>[3x]GVLMDEGAVLTLAADLSSATLDISKQW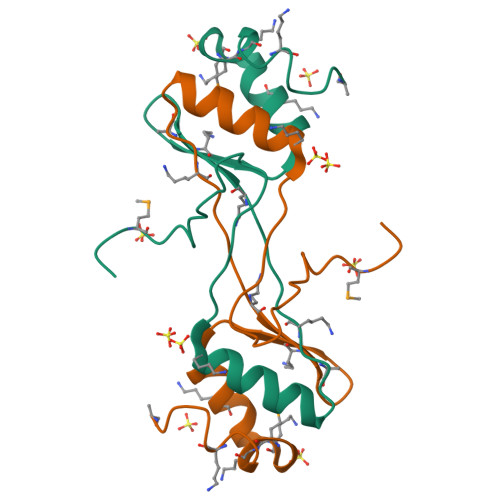SNVFNILRENDFEPKFLCEVKLAFKCDGEIKTFSDLQSLRKFASQKSSMKELLKDVLPQKE>MMKPEDVIKEQCARAKVVAELWHGFTGGAPKAALENLVVEFNKAQQGRCVRPVPQGGYRDLSTKIKAAFAAGKVPTMAQAFENNIALYLEAKALLPIESLGVKLQGVNLTFLNAVRFGGVVYGVPFNKSIQVLYYNKDLLKKHGVPVPATLEEFVAAAKKLSRAEGGPVYWFQPDASTFAYFFFNLGGSYLKDGKLVLNSKEAVEALTLLQNGVKEGWAKPITSGYINQNLGSGPYAFSVDTSAGYTYYLRAAKFDLGVATLPGRTKGQPGYGLVQGTNLVVFRQASKEEQAVAKDFLEF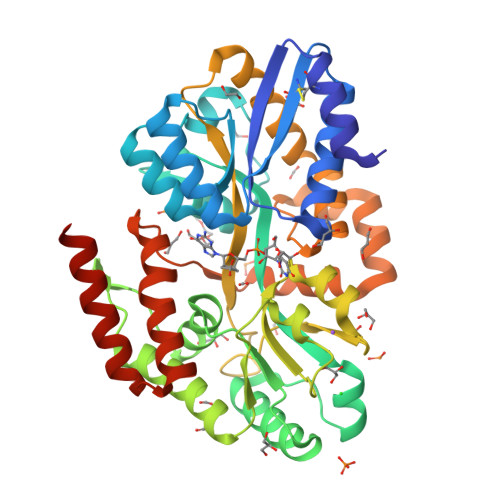VLSPRAQAVFATATGYVPVTEGALKDPVYQAYAAENPDYATIVRQSRYAKFEPALAEWEQIRFDILGQAIKEAILNKADPKAALDRAQKLAEDLLSSRTRHHHHHH[2x]> SPVKVCLIFAGGTGMNVATKLVDLGEAVHCFDTCDKNVVDVHRSVNVTLTKGTRGAGGNRKVILPLVRPQIPALMDTIPEADFYIVCYSLGGGSGSVLGPLITGQLADRKASFVSFVVGAMESTDNLGNDIDTMKTLEAIAVNKHLPIVVNYVPNTQGRSYESINDEIAEKIRKVVLLVNQNHGRLDVHDVANWVRFTDKHNYLIPQVCELHIETTRKDAENVPEAISQLSLYLDPSKEVAFGTPIYRKVGIMKVDDLDVTDDQIHFVINSVGVVEIMKTITDSKLEMTRQ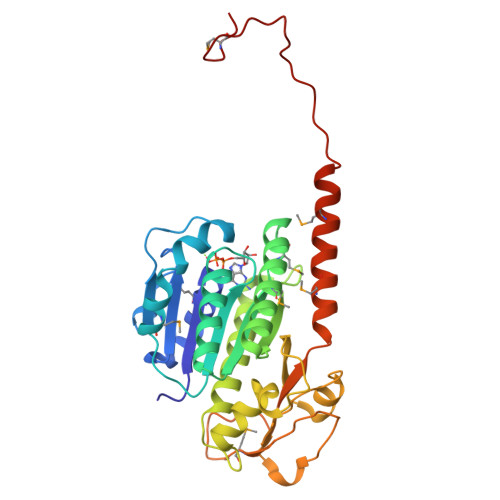QSKFTQRNPIIDADDNVDEDGMVV> KPAAHLIGDPSKQNSLLWRANTDRA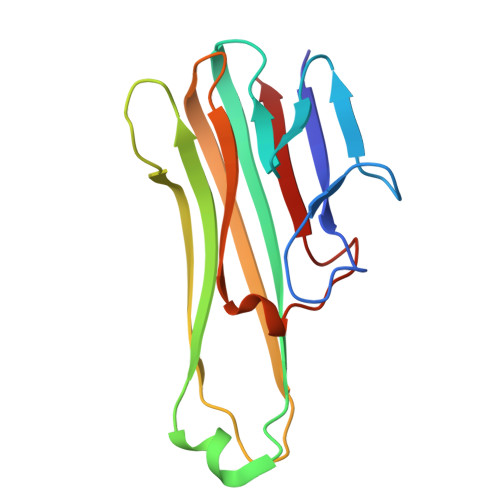FLQDGFSLSNNSLLVPTSGIYFVYSQVVFSGKAYSPKATSSPLYLAHEVQLFSSQYPFHVPLLSSQKMVYPGLQEPWLHSMYHGAAFQLTQGDQLSTHTDGIPHLVLSPSTVFFGAFAL> MGSSHHHHHHSQDPMMEYKIVENGLTYRIGNGASVPISNTGELIKGLRNYGPYEVPSLKYNQIALIHNNQFSSLINQLKSQISSKIDEVWHIHNINISEFIYDSPHFDSIKSQVDNAIDTGVDGIMLVLPEYNTPLYYKLKSYLINSIPSQ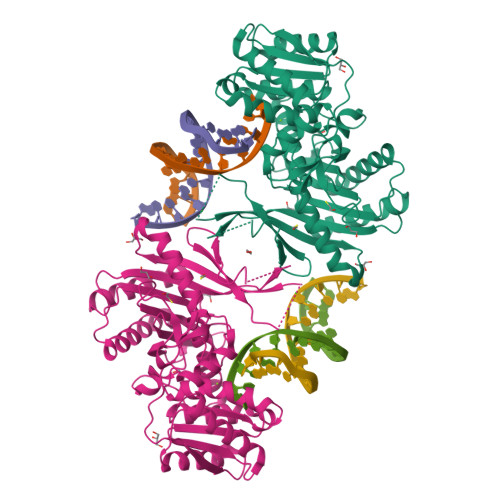FMRYDILSNRNLTFYVDNLLVQFVSKLGGKPWILNVDPEKGSDIIIGTGATRIDNVNLFCFAMVFKKDGTMLWNEISPIVTSSEYLTYLKSTIKKVVYGFKKSNPDWDVEKLTLHVSGKRPKMKDGETKILKETVEELKKQEMVSRDVKYAILHLNETHPFWVMGDPNNRFHPYEGTKVKLSSKRYLLTLLQPYLKRNGLEMVTPIKPLSVEIVSDNWTSEEYYHNVHEILDEIYYLSKMNWRGFRSRNLPVTVNYPKLVAGIIANVNRYGGYPINPEGNRSLQTNPWFL> MALSMTGGQQMGRGSMSRDPLPFFPPLYLGGPEITTENCEREPIHIPGSIQPHGALLTADGHSGEVLQMSLNAATFLGQEPTVLRGQTLAALLPEQWPALQAALPPGCPDALQYRATLDWPAAGHLSLTVHRVGEL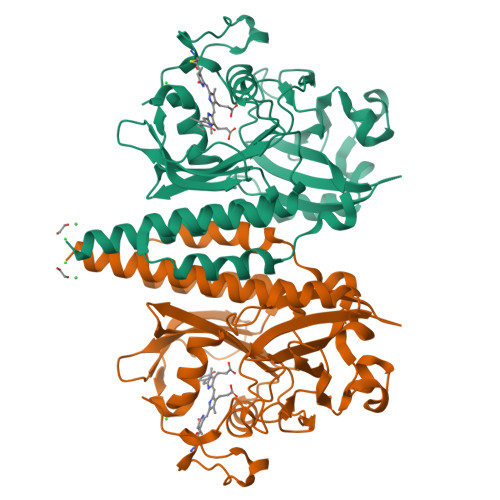LILEFEPTEAWDSTGPHALRNAMFALESAPNLRALAEVATQTVRELTGFDRVMLYKFAPDATGEVIAEARREGLHAFLGHRFPASDIPAQARALYTRHLLRLTADTRAAAVPLDPVLNPQTNAPTPLGGAVLRATSPMHMQYLRNMGVGSSLSVSVVVGGQLWGLIACHHQTPYVLPPDLRTTLESLGRLLSLQVQVKEAHHHHHH> EDKIMSYNAFFWMWVHDMLIDSIKWRDEHGRCINKDKGKTCIKGCNKKCICFQKWVEQKKTEWGKIKDHFRKQKDIPKDWTHDDFLQTLLMKDLLLEIIQDTYGDANEIKRIEALLEQAGVGGIDFAALAGLYTKGFVAEKDTTIDKLLQHEQKEADKCLKTHTDDTCPPQEDRSVARS

Major antigens on the iRBC surface include members of the P. falciparum erythrocyte membrane protein-1 (PfEMP1) family, highly polymorphic and modular proteins composed of DBL (Duffy binding-like) and CIDR (cysteine-rich interdomain region) domains. Adherence of iRBCs to uninfected RBC (known as rosetting) and adherence to the microvasculature (known as sequestration) are thought to be primary causes of morbidity, especially in cerebral and placental malaria. iRBCs adhere due to the binding of PfEMP1 to a variety of endothelial receptors among which are CD36, intercellular adhesion molecule-1 (ICAM-1), and chondroitin sulfate A (CSA). Further analysis of recombinant portions of the MC PfEMP1 molecule identified a 179-residue polypeptide, MC179 (residues 576 to 754), as a minimal portion of the MC CIDR1α domain that retained binding to CD36. We present the structure and analysis of MC179 in the context of the broad sequence diversity of the CIDR domains of the P. falciparum genomes and indicate the insights into overall DBL and PfEMP1 structure that MC179 provides.

MC179 is composed of a bundle of three helices connected by loops and three additional helices. The first helix (H1) of the bundle is joined to the second helix (H2) through a disordered fourteen-residue loop. At the end of the H2 helix there are seventy residues in three smaller helices, a, b, and c, that form the connection to the third helix (H3). The “V-shape” of MC179 is made up of the three-helix bundle and the three helices between the H2 and H3 helices, in the order H1-H2-a-b-c-H3. The H2 and H3 helices also make many contacts with each other and are linked by a conserved disulfide bond, Cys 49-Cys 159, that is observed in the electron density. We directly observed four of the seven cysteines and have evidence that six of the seven cysteines in MC179 are in disulfide bonds. We reasoned that one cysteine had reacted with cystamine (the oxidized form of cysteamine) during protein refolding, which implied that there was one free cysteine in MC179. From comparisons with DBL domains, we concluded that Cys 51 is the single unpaired cysteine in MC179 (see below). The three-helix bundle of MC179 structurally matched each DBL C-terminal three-helix bundle, a region that has also been named “subdomain 3”. In the MC179 crystal, pairs of molecules interact and bury 4300 Å2 of solvent accessible surface area between them.>[2x]MKKILIVDDEKPISDIIKFNLAKEGYDTITAFDGREALSKYEE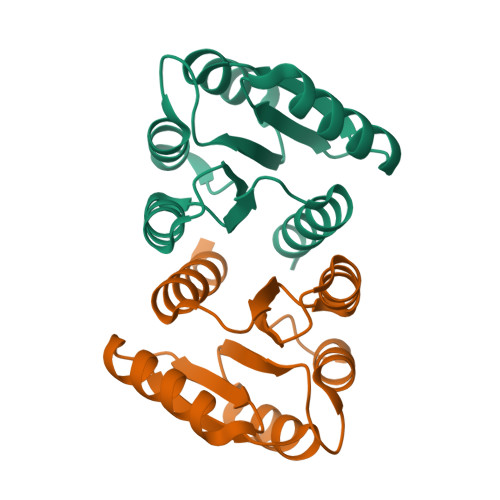ENPDLIILDLMLPELDGLEVAKEVRKNSHVPIIMLSAKDSEFDKVIGLEIGADDYVTKPFSNRELLARVKAHLRRTEN4-(azepan-1-ylcarbonyl)-~{N}-(2-chloranyl-4-methyl-phenyl)-1,2,5-trimethyl-pyrrole-3-sulfonamide 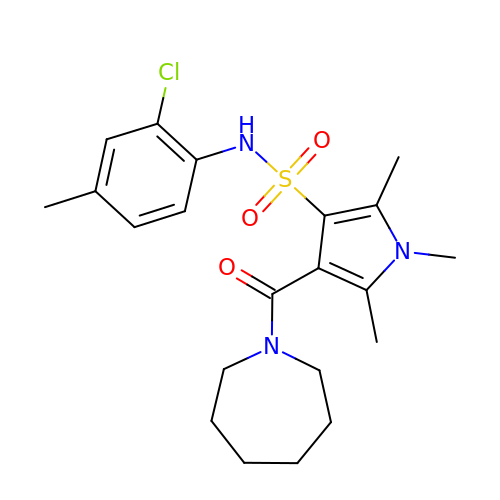| C21 H28 Cl N3 O3 S | QJDVOMDNBMNOMJ-UHFFFAOYSA-N> GGPSFPEPKVVRSQGGLLSLKLSATPTPLAIAGQRATLLTYGGSFPGPTLRVRPRDTVRLTLENRLPEPTNLHWHGLPISPKVDDPFLEIPPGESWTYEFTVPKELAGTFWYHPHLHGRVAPQLFAGLLGALVVESSLDAIPELREAEEHLLVLKDLALQGGRPAPHTPMDWMNGKEGDLVLVNGALRPTLVAQKATLRLRLLNASNARYYRLALQDHPLYLIAADGGFLEEPLEVSELLLAPGERAEVLVRLRKEGRFLLQALPYDRGAMGMMDMGGMAHAMPQGPSRPETLLYLIAPKNPKPLPLPKALSPFPTLPAPVVTRRLVLTEDMMAAR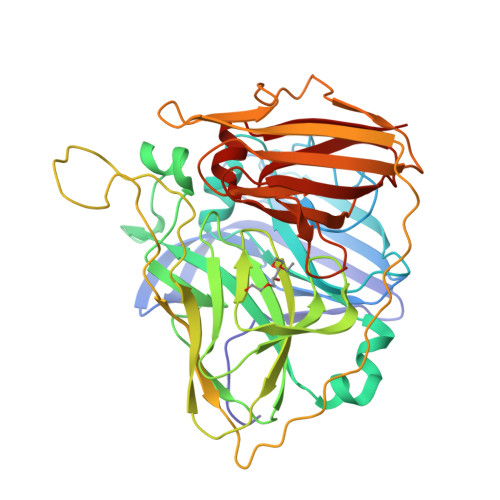FFINGQVFDHRRVDLKGQAQTVEVWEVENQGDMDHPFHLHVHPFQVLSVGGRPFPYRAWKDVVNLKAGEVARLLVPLREKGRTVFHCHIVEHEDRGMMGVLEVG2ALPHA-PROPYL-1ALPHA,25-DIHYDROXYVITAMIN 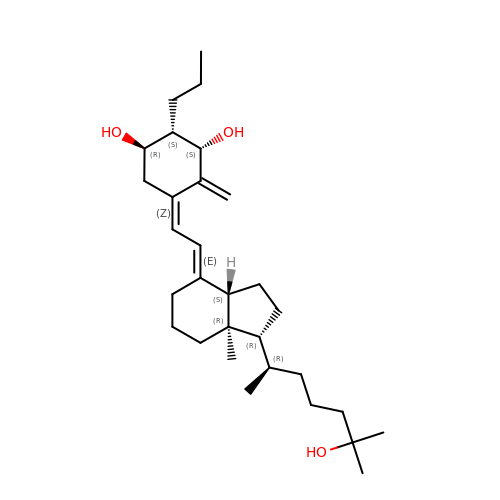D3 | C30 H50 O3 | GMZWKFJQHMQHAO-FMIFKYABSA-N>MMVISEKVRKALNDQLNREIYSSYLYLSMATYFDAEGFKGFVHWMKKQAQEELTHAMKFYEYIYDRGGRVELEAIEKPPSNWNGIKDAFEAALKHEEFVTQSIYNILELASEEKDHATVSFLKWFVDEQVEE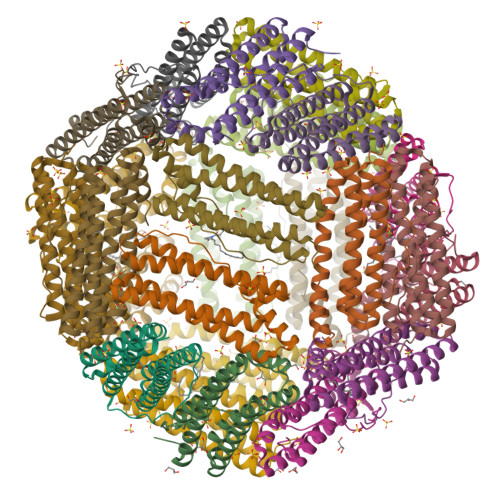EDQVREILDLLEKANGQMSVIFQLDRYLGQRE[8x]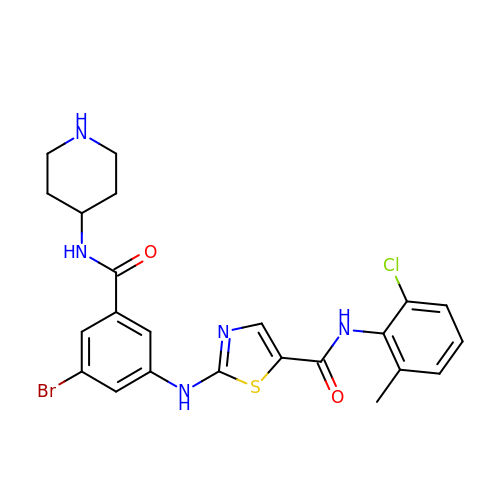2-[[3-bromanyl-5-(piperidin-4-ylcarbamoyl)phenyl]amino]-~{N}-(2-chloranyl-6-methyl-phenyl)-1,3-thiazole-5-carboxamide | C23 H23 Br Cl N5 O2 S | QPHLKSOMHMCVPZ-UHFFFAOYSA-N> ASSLNELNLVQVLEQASNPQHIRSDVQKLAEQQLRQWETQAGFHYLLQSIYLNLSNSLQIRWLAVIQFKNGVDKYWRSTRINAIPKDEKASIRGRLFEMIDEQNNQLCIQNAQASARIARLDFPVEWPTLFEDLENLLNDEIIRKDSVKIYNILMHINQIVKVLGTARIGRCRPAMQSKVPLILPLIVRIYLQSFEEWTTSSNLNYEDLSSLQVSYLALKVLRRIICEGYDRPQTDQSVCDFIKLSVSHFEMLISNHENFKKFDIYEKFIKCLGKLYFNLVTGSPANFILLPCSTQILITYTRLIFDKAPKVYRENSDVTGDFWEQTAIRGLLILKRVINFIHKKGAITLKARSDKLTIDASINKINTEFLNENLITRLVDTLMEWYLRLRPTELENWFMDPEEWINEQMATSYEYQIRPCAENVFQDLMNTFSELLVPYLLKKIENDASKLSNSLDDFLRKDAIYASFQLSASAVSEMVDFDRLLIQVFLPEATNTNISGDELRIIRRRVALIINEWSTVKCSEESKSLCYKLFTNFLTDEDDKVVLLTTVQTVRTMVDDWNFNKDTFQPFLTENVHLLLRKILPSVSLTETRLYVLNTLSDIIIQTKPLISRDLLVEILQIIPNLWEIATNNASEAILANALLRLLRNLVSSLGSQSHLTWDIAIPVVALACDPSSMQYQLLSEDGYELWGMLLQNFSSHDQEFDDKFVELVPFLKYGIETHTEILPTLLEIIKSYALILNPVDFFSNNTFQDIFKQMSKYLLKLREDSFQLVLEIWEI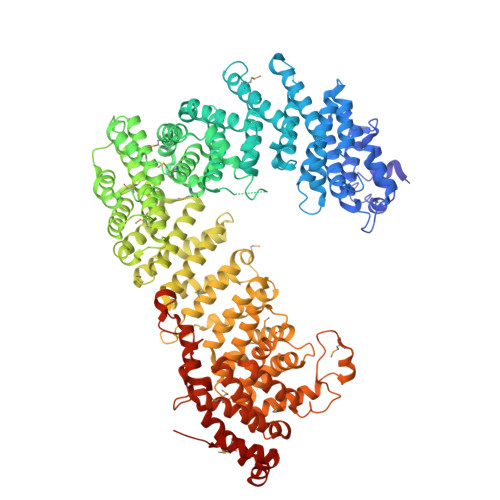LILSNESDYENLLLQKFYETGVLSALFDAIFLEEAPSSYLCSQIIQIIARISYVNPDALMTFLATYHDNLPTSNENARMPESIRKIVSKDQTYDSVVNKLLTGWIVCFRDIFDPKFKKVHILGISSLLRTGLVPILTEFSSIASLWIEMLEEINETNRGDCEKYHLNDIVTEQSIAFHPLTAEQLRYHQLCKNNDPVHNISLKDFISQSMEYLESHLGVERYQEFLKTINPSLLENLQMFLSIQPQEARP> MVTQLKSASEYDSALASGDKLVVVDFFATWCGPSKMIAPMIEKFAEQYSDAAFYKLDVDEVSDVAQKAEVSSMPTLIFYKGGKEVTRV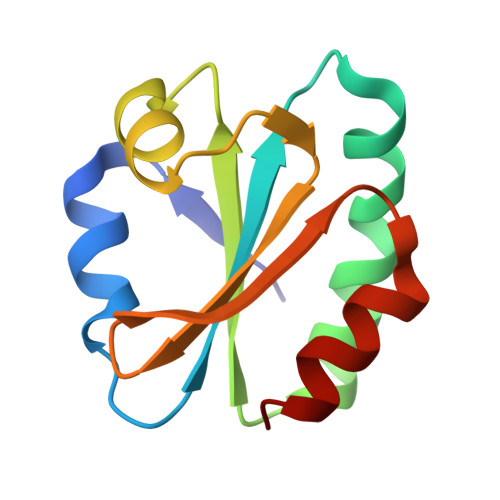VGANPAAIKQAIASNV> KKHVVCQSCDINCVVEAEVKADGKIQTKSISEPHPTTPPNSICMKSVNADTIRTHKDRVLYPLKNVGSKRGEQRWERISWDQALDEIAEKLKKIIAKYGPESLGVSQTEINQQSEYGTLRRFMNLLGSPNWTSAMYMCIGNTAGVHRVTHGSYSFASFADSNCLLFIGKNLSNHNWVSQFNDLKAALKRGCKLIVLDPRRTKVAEMADIWLPLRYGTDAALFLGMINVIINEQLYDKEFVENWCVGFEELKERVQEYPLDKVAEITGCDAGEIRKAAVMFATESPASIPWAVSTDMQKNSCSAIRAQCILRAIVGSFVNGAEILGAPHSDLVPISKIQMHEALPEEKKKLQLGTETYPFLTYTGMSALEEPSERVYGVKYFHNMGAFMANPTALFTAMATEKPYPVKAFFALASNALMGYANQQNALKGLMNQDLVVCYDQFMTPTAQLADYVLPGDHWLERPVVQPNWEGIPFGNTSQQVVEPAGEAKDEYYFIRELAVRMGLEEHFPWKDRLELINYRISPTGMEWEEYQKQYTYMSKLPDYFGPEGVGVATPSGKVELYSSVFEKLGYDPLPYYHEPLQTEISDPELAKEYPLILFAGLREDSNFQSCYHQPGILRDAEPDPVALLHPKTAQSLGLPSGEWIWVETTHGRLKLLLKHDGAQPEGTIRIPHGRWCPEQEGGPETGFSGAMLHNDAMVLSDDDWNLDP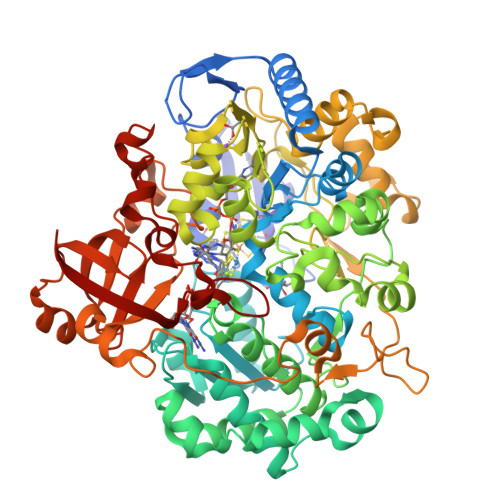EQGLPNLRGGILAKAYKC>[4x]ASAKLPGDFGPPRGEPIHAVLTSPPLVPPPVNRTYPAKVIVELEVVEKEMQISEGVSYTFWTFGGTVPGSFIRVRQGDTVEFHLKNHPSSKMPHNIDLHGVTGPGGGAASSFTAPGHESQFTFKALNEGIYVYHCATAPVGMHIANGMYGLILVEPPEGLPKVDHEYYVMQGDFYTAGKYREKGLQPFDMEKAIDERPSYVLFNGAEGALTGDKALHAKVG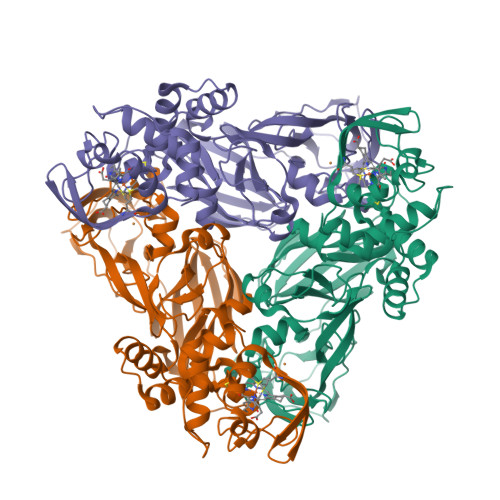ETVRIFVGNGGPNLVSSFHVIGAIFDQVRYEGGTNVQKNVQTTLIPAGGAAVVKFTARVPGSYVLVDHSIFRAFNKGAMAILKIDGAENKLVYSGKELDSVYLGDRAAPNMSAVTKATQASVSGTLTVQDQVQAGRALFAGTCSVCHQGNGAGLPGVFPPLAKSDFLAADPKRAMNIVLHGLNGKIKVNGQEYDSVMPPMTQLNDDEVANILTYVLNSWDNPGGRVSAEDVKKVRAQPAPAKAVAEH>AQYEDGKQYTTLEKPVAGAPQVLEFFSFFCPHCYQFAEVLHISDNVKKKLPEGVKMTKYHVNFMGGDLGKDLTQAWAVAMALGVEDKVT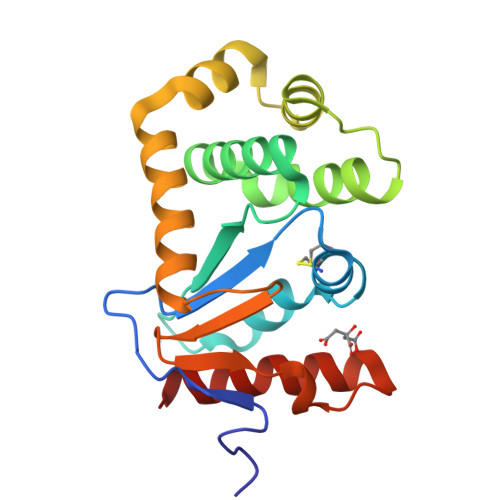VPLFEGVQKTQTIRSASDIRDVFINAGIKGEEYDAAWNSFVVKSLVAQQEKAAADVQLRGVPAMFVNGKYQLNPQGMDTSNMDVFVQQYADTVKYLSEKK[4x]> MLHQLTLAEIARALADKQFSAEELTRTLLGRIRQLDPQLNSFISITDDLAIAQAKAADERRANGENGALLGAPIAHKDLFCTQGVRTSCGSKMLDNFVSPYDAT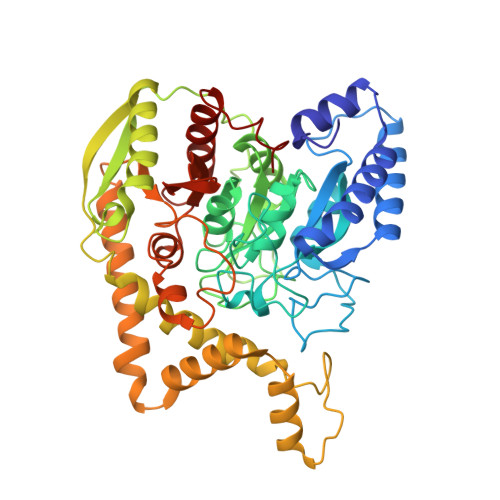VVEKLTAAGAVTLGKLNMDEFAMGSSNQSSHYGAVKNPWSLDRVPGGSSGGSAAAVAARLLPAATGTDTGGSIRQPAALTNLTGIKPTYGRVSRWGMIAYASSLDQGGPLARTAEDCALMLGVMAGFDPKDSTSVEQPVDDYLAALQKPLSGLRIGLPREYFGAGLDSRIADAVLAVVEELKTLGATVKDISLPNMQHAIPAYYVIAPAEASSNLSRFDGVRYGYRCDAPQNLEDLYKRSRAEGFGSEVKNRIMVGTYALSAGYYDAYYLQAQKIRRLIKNDFVSAFAEVDVILGPTTPNPAWKIGEKNDDPVSQYLEDIYTITANLAGLPGLSMPAGFVDGLPVGVQLLAPYFQEGRLLNVAHQYQQVSDWHTRTPAGF> VCPQGKYIHPQDNSICCTKCHKGTYLYNDCPGPGQDTDCRECESGSFTASENHLRHCLSCSKCRKEMGQVEISSCTVD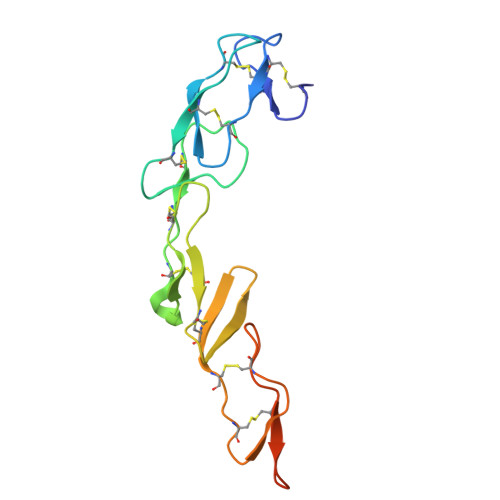RDTVCGCRKNQYRHYWSENLFQCFNCSLCLNGTVHLSCQEKQNTVCTCHAGFFLRENECVSSSN> MAKGTFAKAMPHVFSDEGGYVDHPKDPGGATNMGITLATLSAWEGRKVSKAEVKALTKTKATDIYRENYWNKVAGDDLPAGVDHATLDFAIHSGPARAVKMLQKVVGVDQDGVIGAKTLAAVRKMAADRIINELCDARLAWLKGLGTFST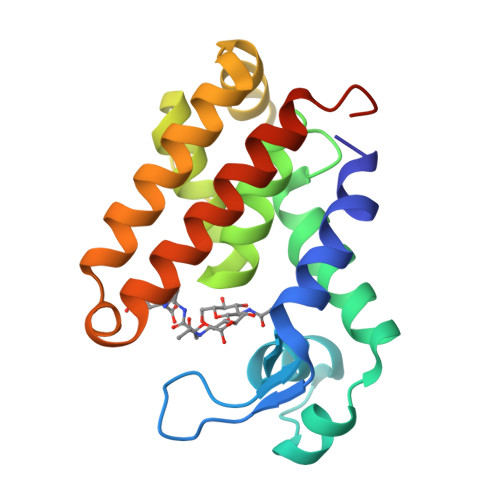FGKGWTSRVSRVRSRALAFSRDSALEHHHHHH> MPEEKQKKSVLEKALKRIEENFGKGSIMILGDETQVQPVEVIPTGSLAIDIATGVGGYPRGRIVEIFGQESSGKTTLALHAIAEAQKMGGVAAFIDAEHALDPVYAKNLGVDLKSLLISQPDHGEQALEIVDELVRSGVVDLIVVDSVAALVPRAEIEGAMGDMQVGLQARLMSQALRKIAGSVNKSKAVVIFTNQIRMKIGVMFGSPETTTGGLALKFYATMRMEVRRGEPIKEGKDVIGNVISVKIVKNKVAPPFKTAQTYIIYGKGIDREYELFN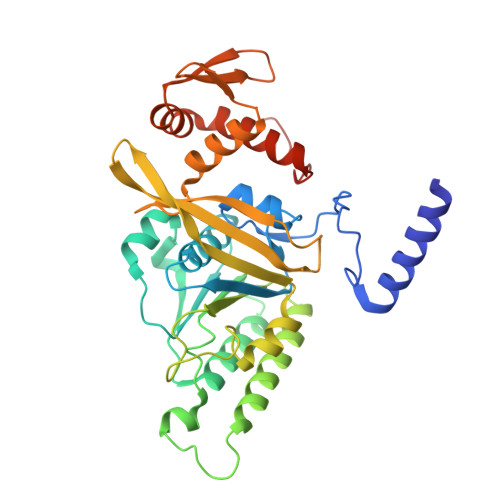IAVNEGIVDRKGSWYYYTTLKGEEVSLGQGSSNAVQFLKDNPEIAGEIERRIREKYGLLSVEKEEQRKEKKSSGEEAS>MAGILEMVARGWKYFSGNFYYFSRTPKTWYSAEQFCISRKAHLTSVSSESEQKFLYKAADGIPHWIGLTKAGSEGDWYWVDQTSFNKEQSRRFWIPGEPNNAGNNEHCANIRVSALKSWNDGPCDNTFLF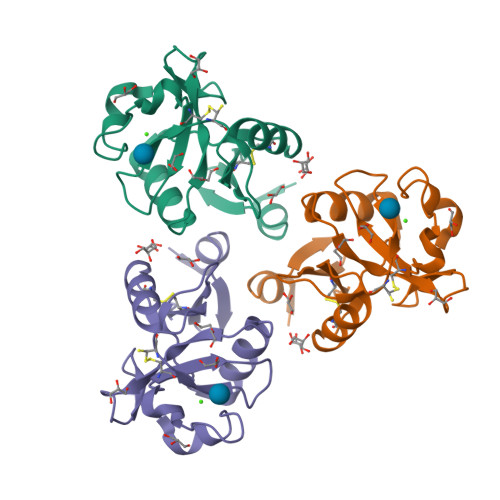ICKRPYVQTTEGTWSHPQFEK[2x]>[2x]MAVLGLQGVRGGVGTTTITAALAWSLQMLGENVLVVDACPDNLLRLSFNVDFTHRQGWARAMLDGQDWRDAGLRYTSQLDLLPFGQLSIEEQENPQHWQTRLSDICSGLQQLKASGRYQWILIDLPRDASQITHQLLSLCDHSLAIVNVDANCHIRLHQQALPDGAHILINNFRIGSQVQDDIYQLWLQ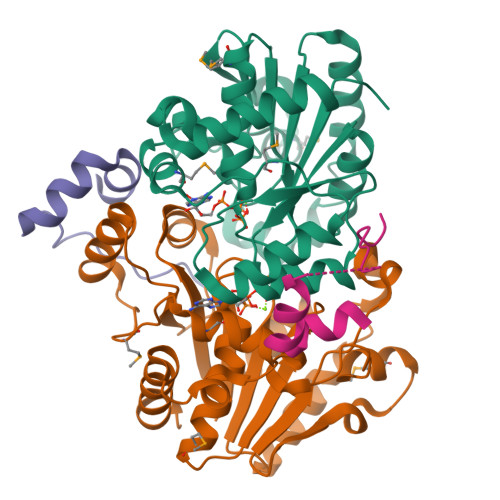SQRRLLPMLIHRDEAMAECLAAKQPVGEYRSDALAAEEILTLANWCLLNYSGLKTPVGSKSAAALEHHHHHH;>MNNNEPDTLPDPAIGYIFQNDIVALKQAFSLPDIDYADISQREQLAAALKRWPLLAEFAQQK[2x]Influenza virus neuraminidase (NA) is an important target for protective antibodies and therapeutic drugs against influenza viruses. NA cleaves off host sialic acids, aiding the release of newly formed virions from infected cells. NA is a mushroom-shaped type II homotetrameric protein. The polypeptide chain of the NA monomeric head folds into six, topologically identical, four-stranded, antiparallel β-sheets which are arranged like the blades of a propeller.

N1/09 hybrid means residues of loops 01 and 23 of N1/2009 grafted to mSN1 (H5N1/2021) scaffold. Twelve dissimilar residues within Loops 01 and 23 of N1/09 were transferred to mSN1 scaffold to form N1/09 hybrid. The N1/09 hybrid showed an 8°C improvement in its melting temperature Tm to 64.4°C compared to the N1/09 protein (56.4°C), while the Tm of the N1/19 hybrid (72.4°C) surpassed the H5N1 mSN1 scaffold donor (68.7°C). In contrast, CD6 bound strongly to the N1/09 hybrid protein, which had a higher Tm of 64.4°C. CD6 also bound strongly to mSN1 scaffold donor. Seven mAbs which did not bind the mSN1 protein but bound N1/09, also bound to the N1/09 hybrid protein, showing their specificity for the transferred loops. To assess whether loop grafting influenced the local or overall structure of the NA, we determined high resolution crystal structures of mSN1, the N1/09 hybrid, and the N1/19 hybrid. Overlay analysis revealed that N1/09 hybrid and N1/19 hybrid were nearly identical in structure to mSN1, with overall RMSDs of <0.25 Å across equivalent Cα atoms upon overlay (Meng et al., 2023). In contrast, the N1/09 and N1/19 hybrids show no noticeable differences between the protomer cavities, all of which closely resemble the wider msN1(ii) conformation, apart from minor, local widening of the rim induced by the substitution of Y344 with an asparagine residue (shown as light-green sticks). Additionally, we observed that the Y344N substitution in the N1/09 and N1/19 hybrids slightly widened the enzymatic cavity compared to msN1. However, N1/09 protein did not induce a cross-reactive response against mSN1, although the N1/09 hybrid did elicit antibodies that inhibited mSN1.

>[2x]MNTQILVFALIAIIPTNADKISAWSHPQFEKGGGGSHHHHHHSSSGSGAHIVMVDAYKPTKGGSGGGGSIINETADDIVYRLTVIIDDRYESLKNLITLRADRLEMIINDNVSTILAGGSGTGSVTLAGNSSLCPISGWAIYSKDNGIRIGSKGDVFVIREPFISCSHLECRTFFLTQGALLNDKHSNGTIKDRSPYRTLMSCPVGEAPSPYNSRFESVAWSASACHDGISWLTIGISGPDNGAVAVVKYNGIITDTIKSWRNNILRTQESECACVNGSCFTVMTDGPSNGQASYKIFKIEKGKVVKSVEMNAPNYHYEECSCYPDAGDIMCVCRDNWHGSNRPWVSFNQNLEYQIGYICSGIFGDNPRPNDKTGSCGPVSSNGANGVKGFSFKYGNGVWIGRTKSISSRNGFEMIWDPNGWTETDSSFSVKQDIVGINEWSGYSGSFVQHPEMTGLDCMRPCFWVELIRGRPKENTIWTSGSSISFCGVNSDTVGWSWPDGAELPFTIDK>GCAGAGU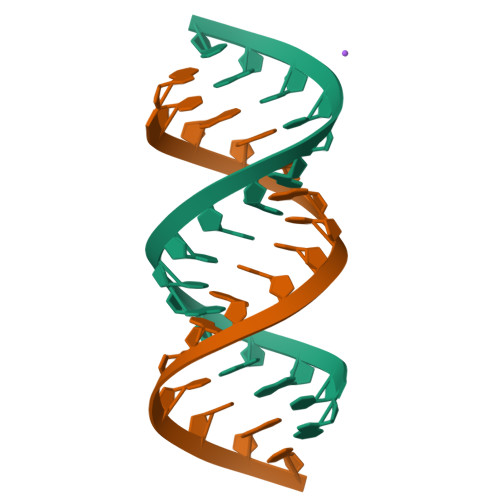UAAAUCUGC[2x]iodoacetic acid | C2 H3 I O2 | 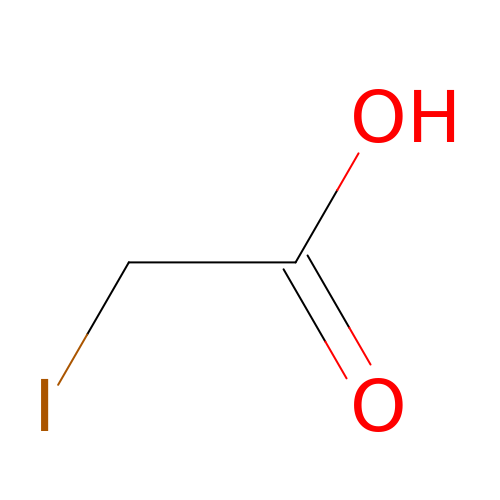JDNTWHVOXJZDSN-UHFFFAOYSA-N> MISNSSAESISAPPNDSTIPHLAIDPFSLDFFDDPYPDQQTLRDAGPVVYLDKWNVYGVARYAEVHAVLNDPTTFCSSRGVGLSDFKKEKPWRPPSLILEADPPAHTRPRAVLSKVLSPATMKTIRDGFAAAADAKVDELLQRGCIDAIADLAEAYPLSVFPDAMGLKQEGREHLLPYAGLVFNAFGPPNELRQTAIERSAPHQAYVNEQCQRPNLAPGGFGACIHAFTDTGEITPDEAPLLVRSLLSAGLDTTVNGIGAAVYCLARFPGELQRL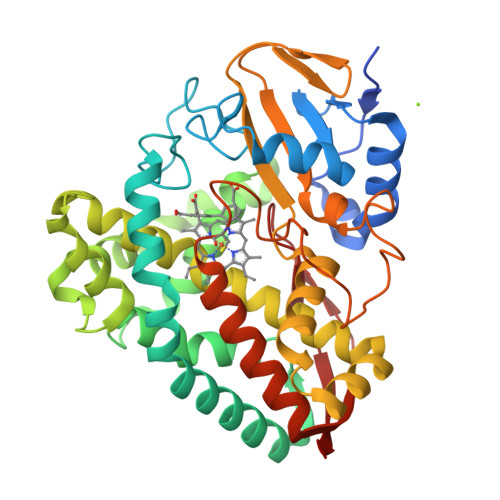RSDPTLARNAFEEAVRFESPVQTVFRTTTREVELGGAVIGEGEKVLMFLGSANRDPRRWSDPDLYDITRKTSGHVGFGSGVHMCVGQLVARLEGEVMLSALARKVAAIDIDGPVKRRFNNTLRGLESLPVKLTPA> MATHTAQTQTHLNFTQIKTAFALYWAL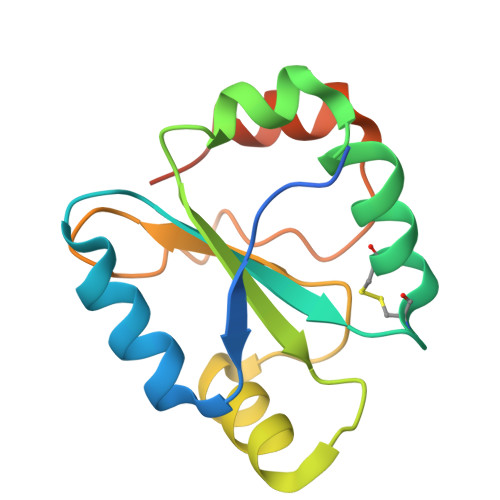LEAQGKPVMLDLYADWCVACKEFEKYTFSDPQVQKALADTVLLQANVTANDAQDVALLKHLNVLGLPTILFFDGQGQEHPQARVTGFMDAETFSAHLRDRQPLEHHHHHH> TRVVYKVPEEQPPNTLIGSLAADYGFPDVGHLYKLEVGAPYLRVDGKTGDIFTTETSIDREGLRECQNQLPGDPCILEFEVSITDLVQNGSPRLLEGQIEVQDINDNTPNFASPVITLAIPENTNIGSLFPIPLASDRDAGPNGVASYELQAGPEAQELFGLQVAEDQEEKQPQLIVMGNLDRERWDSYDLTIKVQDGGSPPRASSALLRVTVLDTNDNAPKFERPSYEAELSENSPIGHSVIQVKANDSDQGANAEIEYTFHQAPEVVRRLLRLDRNTGLITVQGPVDREDLSTLRFSVLAKDRGTNPKSARAQVVVTVKDMNDNAPTIEIRGIGLVTHQDGMANISEDVAEETAVALVQVSDRDEGENAAVTCVVAGDVPFQLRQASETGSDSKKKYFLQTTTPLDYEKVKDYTIEIVAVDSGN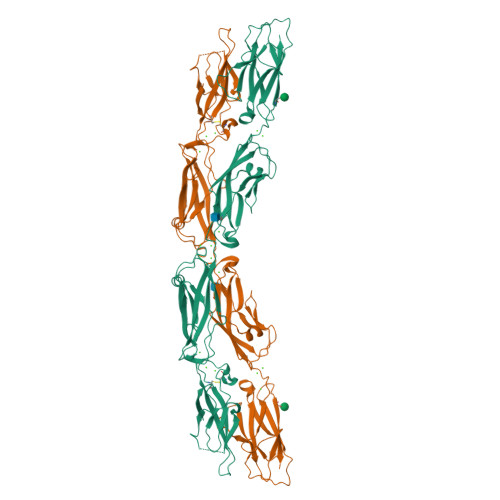PPLSSTNSLKVQVVDVNDNATDPPVGGHHHHHH> GSSHSSANEDMPVERILEAELAVE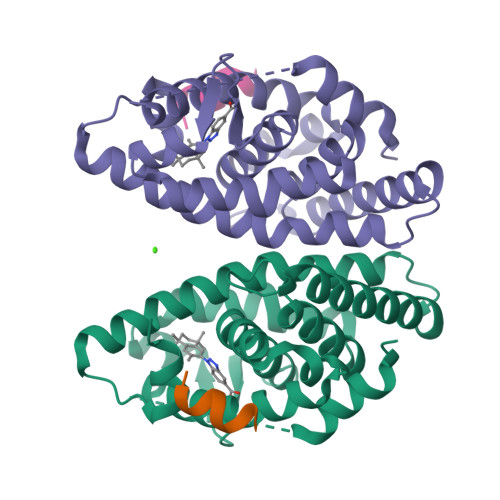PKTETYVEANMGLNPSSPNDPVTNICQAADKQLFTLVEWAKRIPHFSELPLDDQVILLRAGWNELLIASFSHRSIAVKDGILLATGLHVHRNSAHSAGVGAIFDRVLTELVSKMRDMQMDKTELGCLRAIVLFNPDSKGLSNPAEVEALREKVYASLEAYCKHKYPEQPGRFAKLLLRLPALRSIGLKCLEHLFFFKLIGDTPIDTFLMEMLEAPHQMT;> HKILHRLLQEGS>MSSIKVECVLRENYRCGESPVWEEASQSLLFVDIPSKIICRWDTVSNQVQRVAVDAPVSSVALRQLGGYVATIGTKFCALNWENQSVFVLAMVDEDKKNNRFNDGKVDPAGRYFAGTMAEETAPAVLERHQGSLYSLFPDHSVKKYFDQVDISNGLDWSLDHKIFYYIDSLSYTVDAFDYDLQTGQISNRRIVYKMEKDEQIPDGMCIDAEGKLWVACYNGGRVIRLDPETGKRLQTVKLPVDKTTSCCFGGKDYSEMYVTCARDGLNAEGLLRQPDAGNIFKITGLGVKGIAPYSYAG[2x]

Senescence marker protein-30 (SMP30) is a 34-kDa protein whose tissue levels in the liver, kidney, and lung decrease with aging. Biochemical studies suggested that SMP30 is a gluconolactonase (GNL, EC 3.1.1.17) and requires a divalent metal ion such as Zn2+ and Mn2+ for its gluconolactonase activity. In the ascorbic acid biosynthesis pathway, the ring structure of d-glucuronate is cleaved to generate l-gulonate, and then a γ-lactone ring, which is a basic structural framework of ascorbic acid, is formed from l-gulonate by SMP30/GNL. The crystal structure showed that human SMP30/GNL adopts a six-bladed β-propeller fold, which is similar to those of squid diisopropyl-fluorophosphatase (DFPase), drug resistance protein 35 (Drp35), and paraoxonase (PON).

We found that mouse SMP30/GNL can bind 1,5-AG, glucose, and xylitol to the substrate-binding cavity. One hydroxyl group of d-glucose, OH(1), was coordinated to the divalent metal ion. The hydroxyl groups OH(2), OH(3), and OH(4) faced one side of the inner surface of the substrate-binding cavity, as observed in the mouse SMP30/GNL–1,5-AG complex, and formed hydrogen bonds with Arg101, Asn103, and Glu121. Residues on the opposite inner surface of the substrate-binding cavity (Cys16, Ile202, and Tyr219), however, formed no hydrogen bonds with the bound glucose. Polar amino acid residues (Arg101, Asn103, and Glu121) that form hydrogen bonds with hydroxyl groups of a bound molecule are located at one side of the inner surface of the substrate-binding cavity. On the opposite side of the inner surface, there are fewer polar amino-acid residues (Cys16, Ile202, and Tyr219). Due to this asymmetric arrangement of polar residues in the substrate-binding cavity, substrate/product(-analogue) molecules are placed in a specific manner in the cavity.> MGSRRYDSRTTI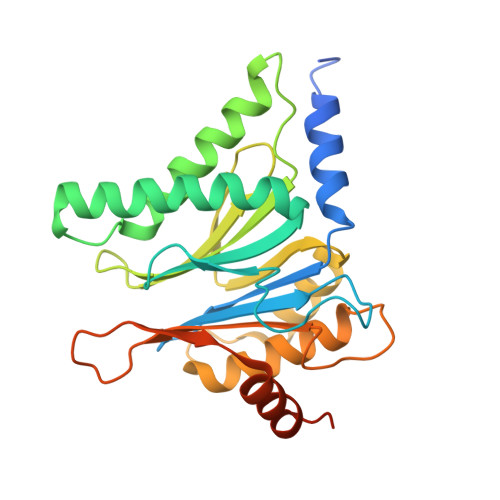FSPEGRLYQVEYALESISHAGTAIGIMASDGIVLAAERKVTSTLLEQDTSTEKLYKLNDKIAVAVAGLTADAEILINTARIHAQNYLKTYNEDIPVEILVRRLSDIKQGYTQHGGLRPFGVSFIYAGYDDRYGYQLYTSNPSGNYTGWKAISVGANTSAAQTLLQMDYKDDMKVDDAIELALKTLSKTTDSSALTYDRLEFATIRKGANDGEVYQKIFKPQEIKDILVKTGITKKDEDEEADEDMK> EQD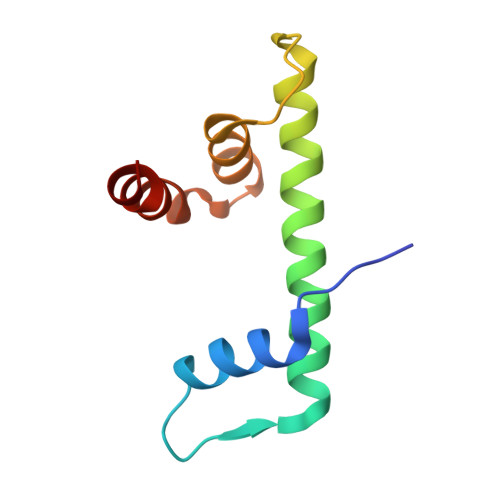IYLPIANVARIMKNAIPQTGKIAKDAKECVQECVSEFISFITSEASERCHQEKRKTINGEDILFAMSTLGFDSYVEPLKLYLQKFR> NAEGDALSALKNSLADPNKVLQSWDATLVTPCTWFHVTCNSDNSVTRVDLGNANLSGQLVMQLGQLPNLQYLELYSNNITGTIPE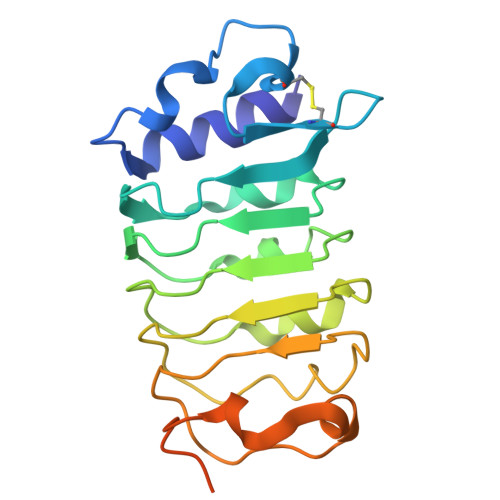QLGNLTELVSLDLYLNNLSGPIPSTLGRLKKLRFLRLNNNSLSGEIPRSLTAVLTLQVLDLSNNPLTGDIPVNGSFSLFTPISFANTKLTPLPASPPPPISPTPPSPAGSHHHHHH>[2x]SNAACSKTNQNSKIATMKGDTITVADFYNEVKNSTASKQAVLSLLVSKVFEKQYGDKV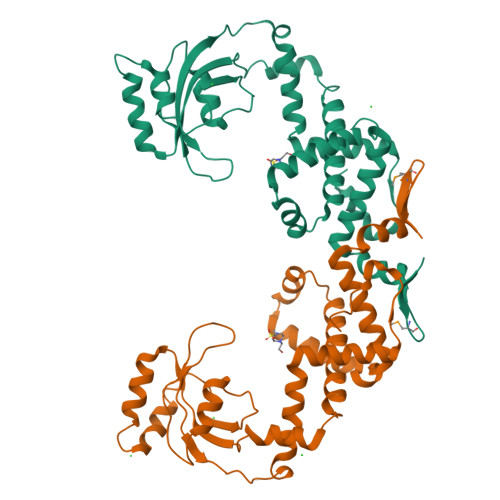SDKEVTKAYNEAAKYYGDSFSSALASRGYTKEDYKKQIRSEKLIEYAVKEEAKKEITDASYKSAYKDYKPEVTAQVIQLDSEDKAKSVLEEAKADGADFAKIAKDNTKGDKTEYSFDSGSTNLPSQVLSAALNLDKDGVSDVIKASDSTTYKPVYYIVKITKKTDKNADWKAYKKRLKEIIVSQKLNDSNFRNAVIGKAFKKANVKIKDKAFSEILSQY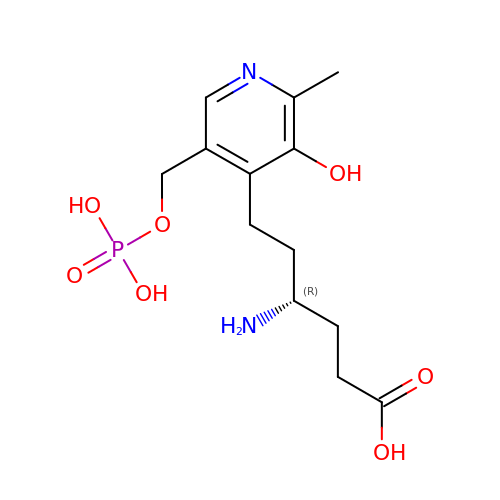(4R)-4-amino-6-{3-hydroxy-2-methyl-5-[(phosphonooxy)methyl]pyridin-4-yl}hexanoic acid | C13 H21 N2 O7 P | CFDRNBOOPNTUHH-SNVBAGLBSA-N> MANTIKVEGYPSMEWPTS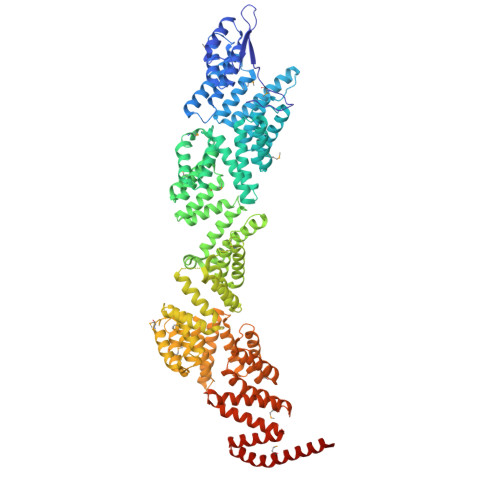LDIPLKASEELVGIDLETDLPDDPTDLKTLLVEESSEKEHWLTIALAYCNHGKTNEGIRLIEMALDVFQNSERASLHTFLTWAHLNLAKGHSLSVETKEHELTQAELNLKDAIGFDPTWIGNMLATVELYYQRGHYDKALETSDLFVKSIHAEDHRSGRQSKPNCLFLLLRAKLLYQKKNYVASLKIFQELLVINPVLQPDPRIGIGLCFWQLKDPKMAIKSWQRALQINSKNTSASILVLLGEFHNSLTDSTNDEVFKETFSKALSDLKNIFSENQNNPVLLTLLQTYHYFKGDFQTVLDIYHHKILKMSPLIAKTVLSESSFWCGRAHYALGDYRKSFIMFQESLKKNEDNLMARLGLGQTQIKSNLLEESIITFENLYKTNESLQELNYILGLLYAGKTLDVKTSKSIPAKELNKLNEKALQYLERYIKLTVAKKNQLIISRVYLVISQLYESQNQYKISLDFLSKALEEMEFVNKDEVPLEILNNLACYHFINGDLTKADNLFEQAKAKVSDMNKSVNITLEYNIARTSEKTNWEKSESIYSQITSSHPSYISARIRNLYIKFAHSKINDSEMNIEINGLLEMNKSDLEMRSFYGWYLKNSEERKNSEKSTSHNKETLVKYNSHDAYALISLANLYVTIARDGKKSRNPKEQEKSKHSYLKAIQLYQKVLQIDPFNVFAAQGVAIIFAESKRLGPALEILRKIRDSLDNEDVQLNLAHCLLEMREFGKAIENYELVLKKFDNERTRPHILNLLGRAWYSRGMKERSVSFFQKALENAKTALELFVQQSAKNKFIHSVKFNIALLQFQIAETLRRSNPKFRTVQQIKDSLEGLEEGLALFKELNDLKEFNMIPKEELEQRIQLGETTMKSALERSLNEQEEFEKDQ>[2x]AHHHHHHGSNLRNKLKLYVITDRRLKPEVESVREALEGGATAIQMRIKNAP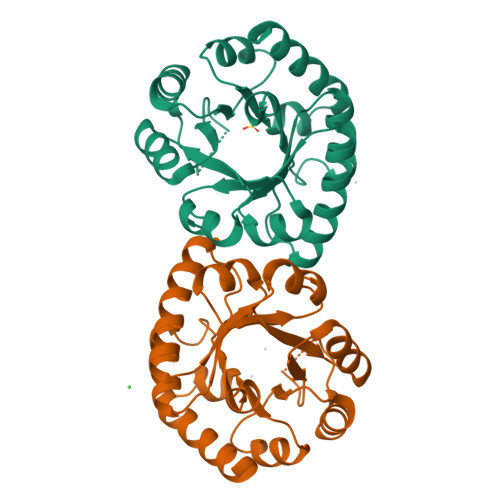TREMYEIGKTLRQLTREYDALFFVDDRVDVALAVDADGVQLGPEDMPIEVAKEIAPNLIIGASVYSLEEALEAEKKGADYLGAGSVFPTKTKEDARVIGLEGLRKIVESVKIPVVAIGGINKDNAREVLKTGVDGIAVISAVMGAEDVRKATEELRKIVEEVLG> MPGSDYKDHDGDYKDHDIDYKDDDDKAAKGSELSERIESFVETLKRGGGPRSSEEMARETLGLLRQIITDHRWSNAGELMELIRREGRRMTAAQPSETTVGNMVRRVLKIIREEYGRLHGRSDESDQQESLHKLLTSGGLNEDFSFHYAQLQSNIIEAINELLVELEGTMENIAAQALEHIHSNEVIMTIGFSRTVEAFLKEAARKRKFHVIVAECAPFCQGHEMAVNLSKAGIETTVMTDAAIFAVMSRVNKVIIGTKTILANGALRAVTGTHTLALAAKHHSTPLIVCAPMFKLSPQFPNEEDSFHKFVAPEEVLPFTEGDILEKVSVHCPVFD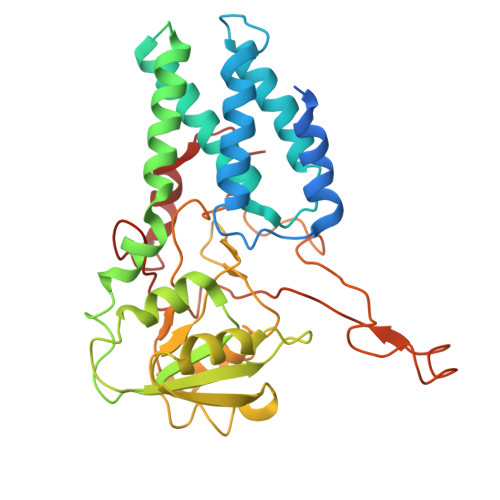YVPPELITLFISNIGGNAPSYIYRLMSELYHPDDHVL> MDLLAELQWRGLVNQTTDEDGLRKLLNEERVTLYCGFDPTADSLHIGHLATILTMRRFQQAGHRPIALVGGATGLIGDPSGKKSERTLNAKETVEAWSARIKEQLGRFLDFEADGNPAKIKNNYDWIGPLDVITFLRDVGKHFSVNYMMAKESVQSRIETGISFTEFSYMMLQAYDFLRLYETEGCRLQIGGSDQWGNITAGLELIRKTKGEARAFGLTIPLVTKADGTKFGKTESGTIWLDKE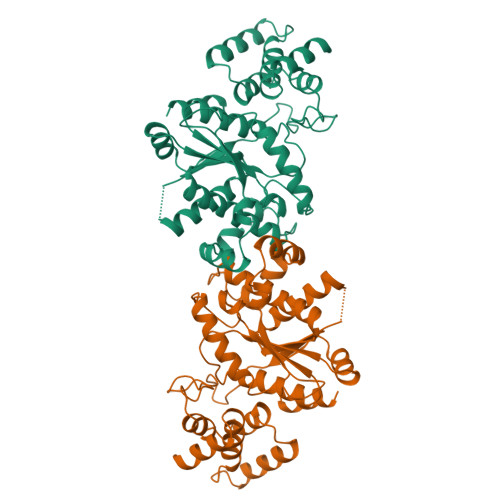KTSPYEFYQFWINTDDRDVIRYLKYFTFLSKEEIEALEQELREAPEKRAAQKTLAEEVTKLVHGEEALRQAIRISEALFSGDIANLTAAEIEQGFKDVPSFVHEGGDVPLVELLVSAGISPSKRQAREDIQNGAIYVNGERLQDVGAILTAEHRLEGRFTVIRRGKKKYYLIRYA> GSMSFLGFGGGQPQLSSQQKIQAAEAELDLVTDMFNKLVNNCYKKCINTSYS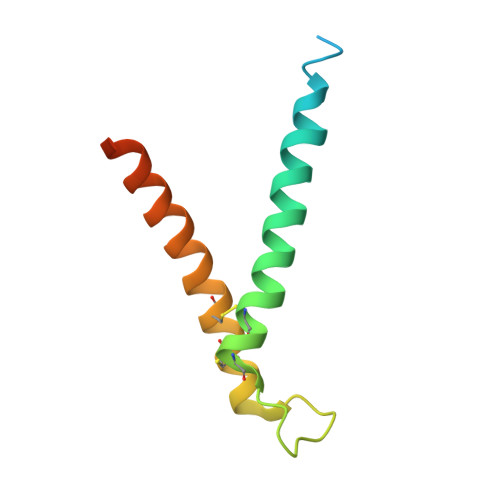EGELNKNESSCLDRCVAKYFETNVQVGENMQKMGQSFNAAGKF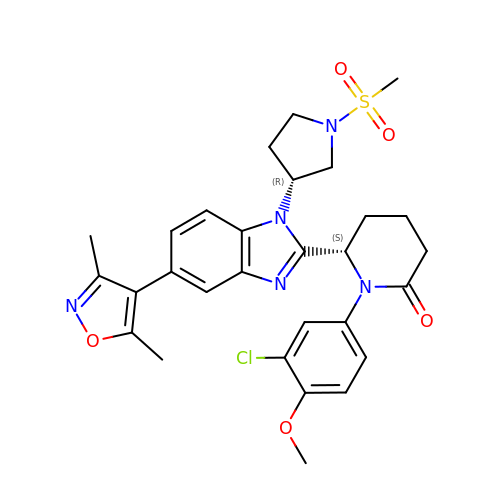(6S)-1-(3-chloranyl-4-methoxy-phenyl)-6-[5-(3,5-dimethyl-1,2-oxazol-4-yl)-1-[(3R)-1-methylsulfonylpyrrolidin-3-yl]benzimidazol-2-yl]piperidin-2-one | C29 H32 Cl N5 O5 S | WMRFYICILGNXCX-BWKNWUBXSA-N> GVFTFQDEYTSTIAPAKLYKALVTDADIIIPKAVETIQSVEIVEGNGGPGTIKKLTFIEGGESKYVLHKIEAIDEANLGYNYSIVGGVGLPDTIEKISFETKLVEGANGGSIGKVTIKIET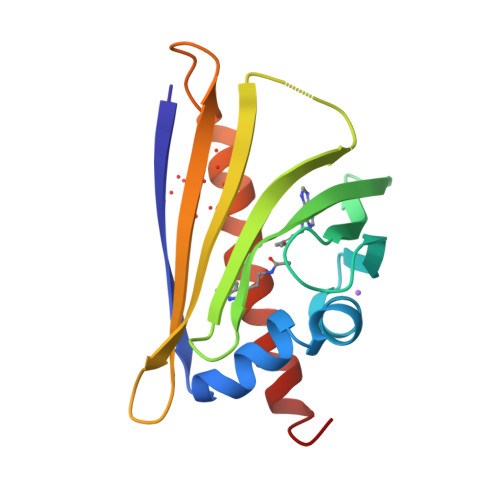KGDAQPNEEEGKAAKARGDAFFKAIESYLSAHPDY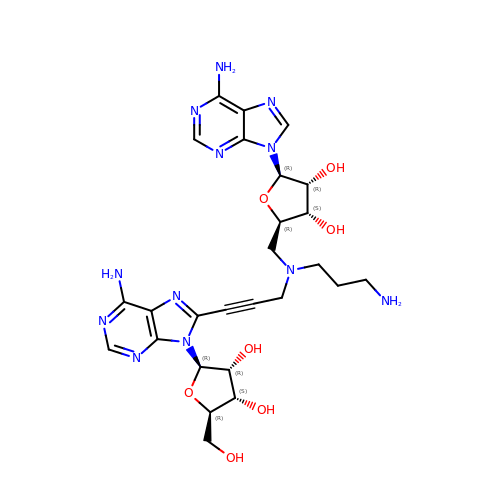(2~{R},3~{R},4~{S},5~{R})-2-(6-aminopurin-9-yl)-5-[[3-[6-azanyl-9-[(2~{R},3~{R},4~{S},5~{R})-5-(hydroxymethyl)-3,4-bis(oxidanyl)oxolan-2-yl]purin-8-yl]prop-2-ynyl-(3-azanylpropyl)amino]methyl]oxolane-3,4-diol | C26 H34 N12 O7 | WXECJKFATFMCJP-DQSURDJZSA-N>NADNYKNVINRTGAPQYMKDYDYDDHQRFNPFFDLGAWHGHLLPDGPNTMGGFPGVALLTEEYINFMASNFDRLTVWQDGKKVDFTLEAYSIPGALVQKLTAKDVQVEMTLRFATPRTSLLETKITSNKPLDLVWDGELLEKLEAKEGKPLSDKTIAGEYPDYQRKISATRDGLKVTFGKVRATWDLLTSGESEYQVHKSLPVQTEINGNRFTSKAHINGSTTLYTTYSHLLTAQEVSKEQMQIRDILARPAFYLTASQQRWEEYLKKGLTNPDATPEQTRVAVKAIETLNGNWRSPGGAVKFNTVT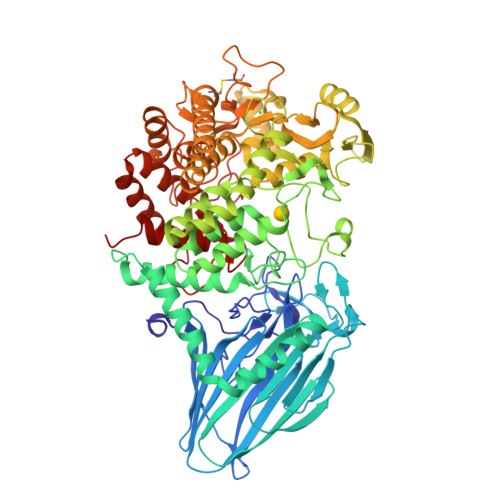PSVTGRWFSGNQTWPWDTWKQAFAMAHFNPDIAKENIRAVFSWQIQPGDSVRPQDVGFVPDLIAWNLSPERGGDGGNWNERNTKPSLAAWSVMEVYNVTQDKTWVAEMYPKLVAYHDWWLRNRDHNGNGVPEYGATRDKAHNTESGEMLFTVKKGDKEETQSGLNNYARVVEKGQYDSLEIPAQVAASWESGRDDAAVFGFIDKEQLDKYVANGGKRSDWTVKFAENRSQDGTLLGYSLLQESVDQASYMYSDNHYLAEMATILGKPEEAKRYRQLAQQLADYINTCMFDPTTQFYYDVRIEDKPLANGCAGKPIVERGKGPEGWSPLFNGAATQANADAVVKVMLDPKEFNTFVPLGTAALTNPAFGADIYWRGRVWVDQFWFGLKGMERYGYRDDALKLADTFFRHAKGLTADGPIQENYNPLTGAQQGAPNFSWSAAHLYMLYNDFFRKQ[2x]>SEKPAFSVLRNETSQAQYKQPVTFNDKLSDANDDFQIKTGYFTCKVPGVYYFVFHASSEGRLCLRLKSTSAPPVSLSFCDFNSKSVSLVVSGGAVLTLLKGDKVWIEPFAGDGGV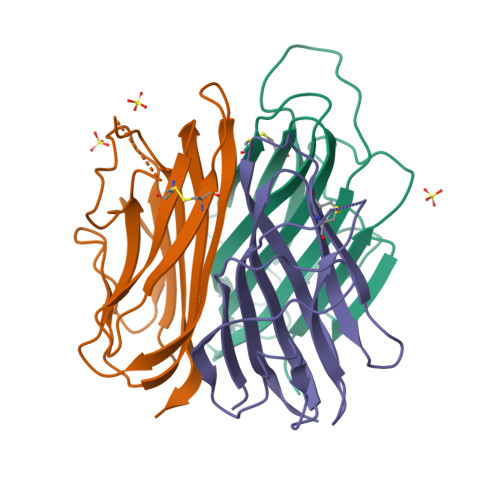GQMPKRLYAVFNGFLIYRN[3x]> MSILTRWLLIPPVNARLIGRYRDYRRHGASAFSATLGCFWMILAWIFIPLEHPRWQRIRAEHKNLYPHINASRPRPLDPVRYLIQTCWLLIGASRKETPKPRRRAFSGLQNIRGRYHQWMNELPERVSHKTQHLDEKKELGHLSAGARRLILGIIVTFSLILALICVTQPFNPLAQFIFLMLLWGVALIVRRMPGRFSALMLIVLSLTVSCRYIWWRYTSTLNWDDPVSLVCGLILLFAETYAWIVLVLGYFQVVWPLNRQPVPLPKDMSLWPSVDIFVPTYNEDLNVVKNTIYASLGIDWPKDKLNIWILDDGGR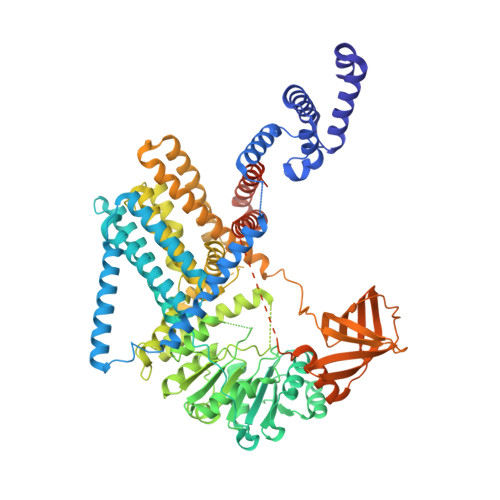EEFRQFAQNVGVKYIARTTHEHAKAGNINNALKYAKGEFVSIFDCDHVPTRSFLQMTMGWFLKEKQLAMMQTPHHFFSPDPFERNLGRFRKTPNEGTLFYGLVQDGNDMWDATFFCGSCAVIRRKPLDEIGGIAVETVTEDAHTSLRLHRRGYTSAYMRIPQAAGLATESLSAHIGQRIRWARGMVQIFRLDNPLTGKGLKFAQRLCYVNAMFHFLSGIPRLIFLTAPLAFLLLHAYIIYAPALMIALFVLPHMIHASLTNSKIQGKYRHSFWSEIYETVLAWYIAPPTLVALINPHKGKFNVTAKGGLVEEEYVDWVISRPYIFLVLLNLVGVAVGIWRYFYGPPTEMLTVVVSMVWVFYNLIVLGGAVAVSVESKQVRRSHRVEMTMPAAIAREDGHLFSCTVQDFSDGGLGIKINGQAQILEGQKVNLLLKRGQQEYVFPTQVARVMGNEVGLKLMPLTTQQHIDFVQCTFARADTWALWQDSYPEDKPLESLLDILKLGFRGYRHLAEFAPSSVKGIFRVLTSLVSWVVSFIPRRPERSETAQPSDQALAQQGSARSSGRTGLEFEEFYPYDVPDYAADYKDDDDKRS>MSRKRNRNRSVQVAKATSEQLNVSRMRMSEQGTFALAKVQVDSERMKAEEIRWPHLIGTAESMKQDATVATGLDMLYTFVEKAFKDFKVIPGESEESKKAAKFIEYCLKNMEGQTLRQFARDAATFNEYGLSVVEKVYTQIAVGEYVGKYKVKNLAFRPQASLSRTNPIVYNSDGSAIVGIKQSLSAFQNYTASEIGVGGVSTRMSDVIIPISRVMLMNTGGSSSQALGVSPLVGCYRAWREKILIENLEVVGATKDMGGVIELKIPSQILNKAAMDPSSPEADMVRGLMSDAANAHSGEQSFFMLPSDTKDNAPQYSMTLKGIDGMGKQYSTAQLISDRKKSILDRLGAGFINVGNDKGGSYNLSESKQTIHTQFVQRVNEIILEALNENLLPQLLALNDIRLPETEMPYVKAGEIVDVDMEGFSKAIQRIGAVGYLPKTPKVINRVLEVLGIDEKIEEDISQEELMKLLGEDTSRAGDGMTKGSSGNGTGKISASRDNSAANLDN[2x];>[2x]MTNEQVIELVRVLLGGITTEEISDQTIIFFWTKWKLTYDLDNRPEKIPAALYNTVVDCVRWLIVQEVSSGNSSIRERFEKIGDETISVKGGSSWESWKDFLDWLELNPDYIDPSLAFNSSLVIIGGVRKDEFFRVKNNPNSYNGFMEQGVYPTPAIPKQSAWPCTAARRSPWMVR;> MARAYSLLSSRNRLIPRVEVQCRKREWVKTDPDSPFLNGGREVLYTPFTAVECTVQPMRGKAIRDQNNQLMIGGEEDYDSYTVYSETLLFRAREGTEHLSDQMLLPDSGGGQTWFTVMKADMYPSSGVPRYRYYLIAVPVGTEGGL;> MALPLDFTNSDVVMGALTKAVGRLCLDVTGYDVVEADETIPKPEGPYILVDLSLLTPLDWATNEVVDEDGVVHTAHNYTASYTLTAYRGKPHWALSRVHQAFGLPFLREKYFPTGSPYAYSSTSNIARMRVPLNQQMFENRARTIVTFNATFVEKDLGTFEDIEHIIIGIDVDNPSGPPIGIGADYDKGVKPGGDDPGLPPKPNPPIVYHDAIAQVCMATPVIDKPALISDKTGE;>[2x]MLNQSKILTLQAYDPAKVLVFIGGQRVSGFAADTKIVITRNNDNISVHAGVDGEISNALSRDNTGVMTLSLQNTAKWNGYLAQWQRQANVTGLIYLPVQVEGSQGLSLNTIGWIQKQPDLSYGTEVGQMDWEIGVLDAWLSPDQIQGIAAGITGLLGLDQ;>[2x]MAEYQDKVVDVEVSLGTQPIDTVGFETPMFLAMHGNFPERIRFYVSTAGMVADGFAVGSP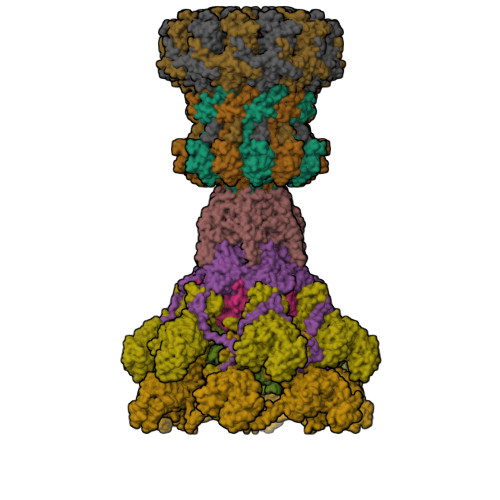AYQFATNAFAGNFAPQRVAIGRMSIDSSKVDFTGTTNTEQVVVNITLNKVVKAVKINVLPGNTPAQIATALADAVTADADLTGKATAVATGTYVTVTAVSPNVVSVGKGAGVYKIVNESSETVATVLPSVIAENHNWYFLATEARSDADIVAAAEFAKANYKLHIYNSTDVDAYAPENSAASVFDTLKSLSYDSLGTSDAGADVDFTEGSVIGAMAANDPSYGDSLHLKTMPGMVPFAGSDTQRSNAWSRNANIYRGLYGGGSYIEGKTSSGQYVDVIRFSHWVKFRMEESVFAYMKRRSDMGLSMKMSDEDLPVLKSVLMNNPINIGIRNGGILTGYDTENKVSYDPTIIIPKRANIPTNDLAARILRDVKVELVYNNSLHYVKIRASVVLDRPAGQSTNAQTPMSSSAVGV>CPRFLKVKNWETEVVLTDTLHLKSTLETGCTEYICMGSIMHPSQHARRPEDVATKDQLFPLAKEFIDQYYSSIKRFGSKAHMERLEEVNKEIDTTSTYQLKDTELIYGAKHAWRNASRCVGRIQWSKLQVFDARDCTTAHGMFNYICNHVKYATNKGNLRSAITIFPQRTDGKHDFRVWNSQLIRYAGYKQPDGSTLGDPANVQFTEICIQQGWKPPRGRFDVLPLLLQANGNDPELFQIPPELVLEVPIRHPKFEWFKDLGLKWYGLPAVSNMLLEIGGLEFSACPFSGWYMGTEIGVRDYCDNSRYNILEEVAKKMNLDMRKTSSLWKDQALVEINIAVLYSFQSDKVTIVDHHSATESFIKHMENE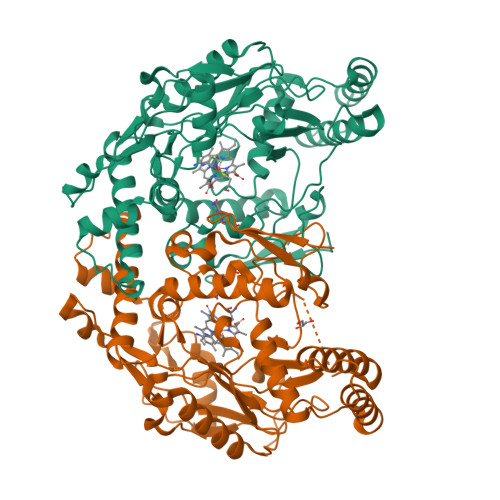YRCRGGCPADWVWIVPPMSGSITPVFHQEMLNYRLTPSFEYQPDPWNTHVWKLV[4x]> QSDTHIFIIMGASGDLAKKKIYPTIWWLFRDGLLPENTFIVGYARSRLTVADIRKQSEPFFKATPEEKLKLEDFFARNSYVAGQYDDAASYQRLNSHMNALHLGSQANRLFYLALPPTVYEAVTKNIHESCMSQIGWNRIIVEKPFGRDLQSSDRLSNHISSLFREDQIYRIDHYLGKEMVQNLMVLRFANRIFGPIWNRDNIACVILTFKEPFGTEGRGGYFDEFGIIRDVMQNHLLQMLCLVAMEKPASTNSDDVRDEKVKVLKCISEVQANNVVLGQYVGNPDGEGEATKGYLDDPTVPRGSTTATFAAVVLYVENERWDGVPFILRCGKALNERKAEVRLQFHDVAGDIFHQQCKRNELVIRVQPNEAVYTKMMTKKPGMFFNPEESELDLTYGNRYKNVKLPDAYERLILDVFCGSQMHFVRSDELREAWRIFTPLLHQIELEKPKPIPYIYGSRGPTEADELMKRVGFQYEGTYKWVN

Glucose-6-phosphate dehydrogenase (G6PD) catalyzes the first and rate-limiting reaction in the PPP; the oxidation of glucose-6-phosphate (G6P) to 6-phosphogluconolactone with concomitant reduction of nicotinamide adenine dinucleotide phosphate (NADP+) to NADPH. G6PD is a major source of cellular NADPH and has a primary role in controlling the metabolic flux through the PPP. G6PD is catalytically active as a homodimer or homotetramer. Each monomer has one G6P binding site (i.e., the catalytic site) and can bind two NADP+ molecules; one is close to the G6P binding site, and the other is the structural NADP+ binding site.

To test the hypothesis that K95/97 ubiquitylation is affected by K89 acetylation-dependent structural changes, we determined the crystal structure of K89-acetylated G6PD. AcK89 G6PD was crystallized in the F222 space group with one protein molecule and structural NADP+ within the asymmetric unit, and the structure was solved to a resolution of 2.46 Å (statistics of data collection and model refinement are listed in Supplementary Table 3). Similarly, the dimeric structures of AcK89 (obtained by symmetry operations) and WT G6PD were essentially identical (Cα RMSD value of 0.35 Å). In contrast, notable local conformational changes were found around residue AcK89, which was rotated by ~180° relative to non-acetylated K89. This conformational change resulted in the partial unwinding of helix αb’ and rotation of residues E94–K97 by ~45° relative to the helix axis. Thus, according to the crystal structure of AcK89, ubiquitylation of K95/97 may be promoted by K89 acetylation-dependent local conformational changes. Western blot analysis found that the ubiquitylation level of AcK89 G6PD was higher, relative to pWT, AcK95, and AcK97 G6PD, suggesting that K89 acetylation promotes the ubiquitylation of G6PD. Next, we introduced K95R, K97R, or K95/97R mutations into pWT and AcK89 G6PD and verified that these mutations have no effect on Vmax. Mutation of either K95 or K97 to arginine reduced the level of AcK89 G6PD ubiquitylation considerably, showing that K89 acetylation promotes the ubiquitylation of G6PD on residues K95/97. According to the measured kinetic parameters, AcK386, AcK408, AcK432, and AcK497 G6PD had 30–70% lower enzymatic efficiency (Kcatapp/KMapp) compared to WT G6PD, AcK403 displayed significantly lower activity, and AcK89 G6PD displayed similar Kcatapp/KMapp for G6P, but 2-fold higher catalytic efficiency for NADP+. Residue K89 is not part of the active site or other functionally important elements, yet, it is highly conserved from E. coli to mammals.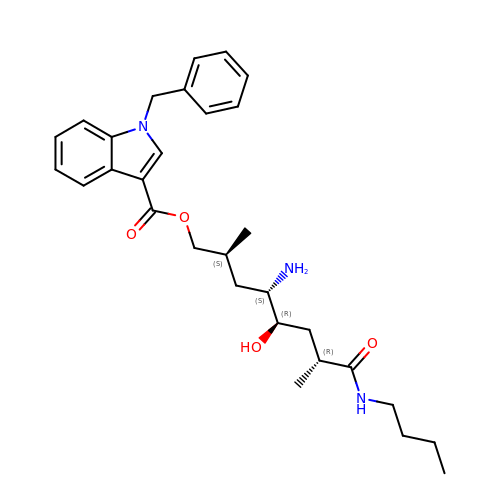(2S,4S,5R,7R)-4-AMINO-8-(BUTYLAMINO)-5-HYDROXY-2,7-DIMETHYL-8-OXOOCTYL 1-BENZYL-1H-INDOLE-3-CARBOXYLATE | C30 H41 N3 O4 | XZLFXZZCYRJLTI-PGVSFRRCSA-N>[4x]MQGSVTEFLKPRLVDIEQVSSTHAKVTLEPLERGFGHTLGNALRRILLSSMPGCAVTEVEIDGVLHEYSTKEGVQEDILEILLNLKGLAVRVQGKDEVILTLNKSGIGPVTAADITHDGDVEIVKPQHVICHLTDENASISMRIKVQRGRGYVPASTRIHSEEDERPIGRLLVDACYSPVERIAYNVEAARVEQRTDLDKLVIEMETNGTIDPEEAIRRAATILAEQLEAFVDLRDVRQPEVKEEKPEFDPILLRPVDDLELTVRSANCLKAEAIHYIGDLVQRTEVELLKTPNLGKKSLTEIKDVLASRGLSLGMRLEN;>MVYSYTEKKRIRKDFGKRPQVLDVPYLLSIQLDSFQKFIEQDPEGQYGLEAAFRSVFPIQSYSGNSELQYVSYRLGEPVFDVQECQIRGVTYSAPLRVKLRLVIYEREAPEGTVKDIKEQEVYMGEIPLMTDNGTFVINGTERVIVSQLHRSPGVFFDSDKGKTHSSGKVLYNARIIPYRGSWLDFEFDPKDNLFVRIDRRRKLPATIILRALNYTTEQILDLFFEKVIFEIRDNKLQMELVPERLRGETASFDIEANGKVYVEKGRRITARHIRQLEKDDVKLIEVPVEYIAGKVVAKDYIDESTGELICAANMELSLDLLAKLSQSGHKRIETLFTNDLDHGPYISETLRVDPTNDRLSALVEIYRMMRPGEPPTREAAESLFENLFFSEDRYDLSAVGRMKFNRSLLREEIEGSGILSKDDIIDVMKKLIDIRNGKGEVDDIDHLGNRRIRSVGEMAENQFRVGLVRVERAVKERLSLGDLDTLMPQDMINAKPISAAVKEFFGSSQLSQFMVQNNPLSEITHKRRISALGPGGLTRERAGFEVRDVHPTHYGRVCPIETPEGPNIGLINSLSVYAQTNEYGFLETPYRKVTDGVVTDEIHYLSAIEEGNYVIAQANSNLDEEGHFVEDLVTCRSKGESSLFSRDQVDYMDVSTQQVVSVGASLIPFLEHD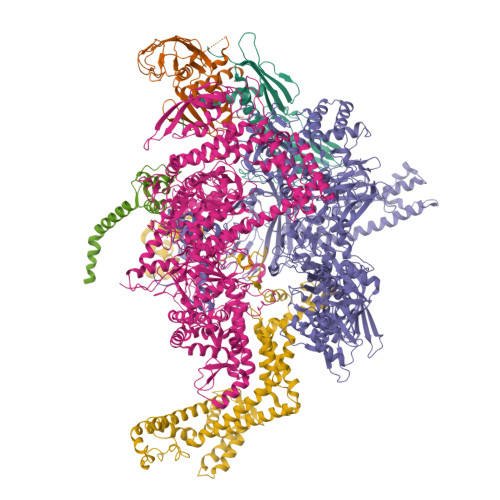DANRALMGANMQRQAVPTLRADKPLVGTGMERAVAVDSGVTAVAKRGGVVQYVDASRIVIKVNEDEMYPGEAGIDIYNLTKYTRSNQNTCINQMPCVSLGEPVERGDVLADGPSTDLGELALGQNMRVAFMPWNGYNFEDSILVSERVVQEDRFTTIHIQELACVSRDTKLGPEEITADIPNVGEAALSKLDESGIVYIGAEVTGGDILVGKVTPKGETQLTPEEKLLRAIFGEKASDVKDSSLRVPNGVSGTVIDVQVFTRDGVEKDKRALEIEEMQLKQAKKDLSEELQILEAGLFSRIRAVLVAGGVEAEKLDKLPRDRWLELGLTDEEKQNQLEQLAEQYDELKHEFEKKLEAKRRKITQGDDLAPGVLKIVKVYLAVKRRIQPGDKMAGRHGNKGVISKINPIEDMPYDENGTPVDIVLNPLGVPSRMNIGQILETHLGMAAKGIGDKINAMLKQQQEVAKLREFIQRAYDLGADVRQKVDLSTFSDEEVMRLAENLRKGMPIATPVFDGAKEAEIKELLKLGDLPTSGQIRLYDGRTGEQFERPVTVGYMYMLKLNHLVDDKMHARSTGSYSLVTQQPLGGKAQFGGQRFGEMEVWALEAYGAAYTLQEMLTVKSDDVNGRTKMYKNIVDGNHQMEPGMPESFNVLLKEIRSLGINIELEDE[2x];>[2x]MKDLLKFLKAQTKTEEFDAIKIALASPDMIRSWSFGEVKKPETINYRTFKPERDGLFCARIFGPVKDYECLCGKYKRLKHRGVICEKCGVEVTQTKVRRERMGHIELASPTAHIWFLKSLPSRIGLLLDMPLRDIERVLYFESYVVIEGGMTNLERQQILTEEQYLDALEEFGDEFDAKMGAEAIQALLKSMDLEQECEQLREELNETNSETKRKKLTKRIKLLEAFVQSGNKPEWMILTVLPVLPPDLRPLVPLDGGRFATSDLNDLYRRVINRNNRLKRLLDLAAPDIIVRNEKRMLQEAVDALLDNGRRGRAITGSNKRPLKSLADMIKGKQGRFRQNLLGKRVDYSGRSVITVGPYLRLHQCGLPKKMALELFKPFIYGKLELRGLATTIKAAKKMVEREEAVVWDILDEVIREHPVLLNRAPTLHRLGIQAFEPVLIEGKAIQLHPLVCAAYNADFDGDQMAVHVPLTLEAQLEARALMMSTNNILSPANGEPIIVPSQDVVLGLYYMTRDCVNAKGEGMVLTGPKEAERLYRSGLASLHARVKVRITEYEKDANGELVAKTSLKDTTVGRAILWMIVPKGLPYSIVNQALGKKAISKMLNTCYRILGLKPTVIFADQIMYTGFAYAARSGASVGIDDMVIPEKKHEIISEAEAEVAEIQEQFQSGLVTAGERYNKVIDIWAAANDRVSKAMMDNLQTETVINRDGQEEKQVSFNSIYMMADSGARGSAAQIRQLAGMRGLMAKPDGSIIETPITANFREGLNVLQYFISTHGARKGLADTALKTANSGYLTRRLVDVAQDLVVTEDDCGTHEGIMMTPVIEGGDVKEPLRDRVLGRVTAEDVLKPGTADILVPRNTLLHEQWCDLLEENSVDAVKVRSVVSCDTDFGVCAHCYGRDLARGHIINKGEAIGVIAAQSIGEPGTQLTMRTFHIGGAASRAAAESSIQVKNKGSIKLSNVKSVVNSSGKLVITSRNTELKLIDEFGRTKESYKVPYGAVLAKGDGEQVAGGETVANWDPHTMPVITEVSGFVRFTDMIDGQTITRQTDELTGLSSLVVLDSAERTAGGKDLRPALKIVDAQGNDVLIPGTDMPAQYFLPGKAIVQLEDGVQISSGDTLARIPQESGGTKDITGGLPRVADLFEARRPKEPAILAEISGIVSFGKETKGKRRLVITPVDGSDPYEEMIPKWRQLNVFEGERVERGDVISDGPEAPHDILRLRGVHAVTRYIVNEVQDVYRLQGVKINDKHIEVIVRQMLRKATIVNAGSSDFLEGEQVEYSRVKIANRELEANGKVGATYSRDLLGITKASLATESFISAASFQETTRVLTEAAVAGKRDELRGLKENVIVGRLIPAGTGYAYHQDRMRRRAAGEAPAAPQVTAEDASASLAELLNAGLGGSDNE;>[2x]ARVTVQDAVEKIGNRFDLVLVAARRARQMQVGGKDPLVPEENDKTTVIALREIEEGLINNQILDVRERQEQQEQEAAELQAVTAIAEGRR;>MEQNPQSQLKLLVTRGKEQGYLTYAEVNDHLPEDIVDSDQIEDIIQMINDMGIQVMEEAPDADDLMLAENTADEDAAEAAAQVLSSVESEIGRTTDPVRMYMREMGTVELLTREGEIDIAKRIEDGINQVQCSVAEYPEAITYLLEQYDRVEAEEARLSDLITGFVDPNAEEDLAPTATHVGSELSQEDLDDDEDEDEEDGDDDSADDDNSIDPELAREKFAELRAQYVVTRDTIKAKGRSHATAQEEILKLSEVFKQFRLVPKQFDYLVNSMRVMMDRVRTQERLIMKLCVEQCKMPKKNFITLFTGNETSDTWFNAAIAMNKPWSEKLHDVSEEVHRALQKLQQIEEETGLTIEQVKDINRRMSIGEAKARRAKKEMVEANLRLVISIAKKYTNRGLQFLDLIQEGNIGLMKAVDKFEYRRGYKFSTYATWWIRQAITRSIADQARTIRIPVHMIETINKLNRISRQMLQEMGREPTPEELAERMLMPEDKIRKVLKIAKEPISMETPIGDDEDSHLGDFIEDTTLELPLDSATTESLRAATHDVLAGLTAREAKVLRMRFGIDMNTDYTLEEVGKQFDVTRERIRQIEAKALRKLRHPSRSEVLRSFLDD[2x]>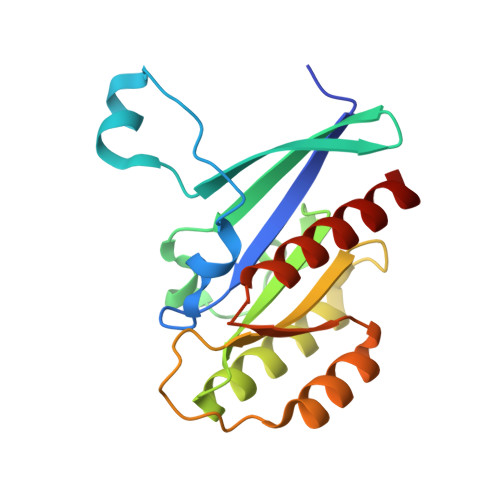 GHMPEYDYLFKLLLIGDSGVGKSCLLLRFADDTYTESYISTIGVDFKIRTIELDGKTIKLQIWDTAGQERFRTITSSYYRGAHGIIVVYDVTDQESYANVKQWLQEIDRYASENVNKLLVGNKSDLTTKKVVDNTTAKEFADSLGIPFLETSAKNATNVEQAFMTMAAEIKKRMG> AEGTRGRSSTARCSLFGSDFVNTFDGSMYSFAGYCSYLLAGGCQKRSFSIIGDFQNGKRVSLSVYLGEFFDIHLFVNGTVTQGDQRVSMPYASKGLYLETEAGYYKLSGEAYGFVARIDGSGNFQVLLSDRYFNKTCGLCGNFNIFAEDDFMTQEGTLTSDPYDFANSWALSSGEQWCERASPPSSSCNISSGEMQKGLWEQCQLLKSTSVFARCHPLVDPEPFVALCEKTLCECAGGLECACPALLEYARTCAQEGMVLYGWTDHSACSPVCPAGMEYRQCVSPCARTCQSLHINEMCQERCVDGCSCPEGQLLDEGLCVESTECPCVHSGKRYPPGTSLSRDCNTCICRNSQWICSNEECPGECLVTGQSHFKSFDNRYFTFSGICQYLLARDCQDHSFSIV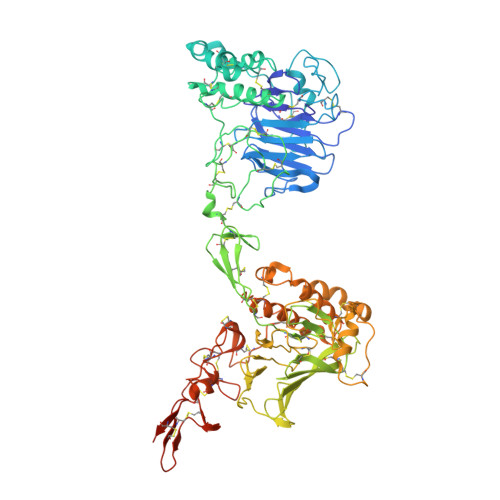IETVQCADDRDAVCTRSVTVRLPGLHNSLVKLKHGAGVAMDGQDVQLPLLKGDLRIQHTVTASVRLSYGEDLQMDWDGRGRLLVKLSPVYAGKTCGLCGNYNGNQGDDFLTPSGLAEPRVEDFGNAWKLHGDCQDLQKQHSDPCALNPRMTRFSEEACAVLTSPTFEACHRAVSPLPYLRNCRYDVCSCSDGRECLCGALASYAAACAGRGVRVAWREPGRCELNCPKGQVYLQCGTPCNLTCRSLSYPDEECNEACLEGCFCPPGLYMDERGDCVPKAQCPCYYDGEIFQPEDIFSDHHTMCYCEDGFMHCTMSGVPGSLLPDAVLSSPLSHRSKR>AMGSATISRRGILVIRHGERVDQVFGKSWLQQCTTADGKYYRPDLNFPRSLPRRSNGIKDFENDPPLSSCGIFQARLAGEALLDSGVRVTAVFASPALRCVQTAKHILEELKLEKKLKIRVEPGIFEWMKWEASKATLTFLTLEELKEANFNVDLDYRPALPRCSLMPAESYDQYVERCAVSMGQIINTCPQDMGITLIVSHSSALDSCTRPLLGLPPRECGDFAQLVRKIPSLGMCFCEENREDGKWDLVNPPVKTLTHGANSVFNWR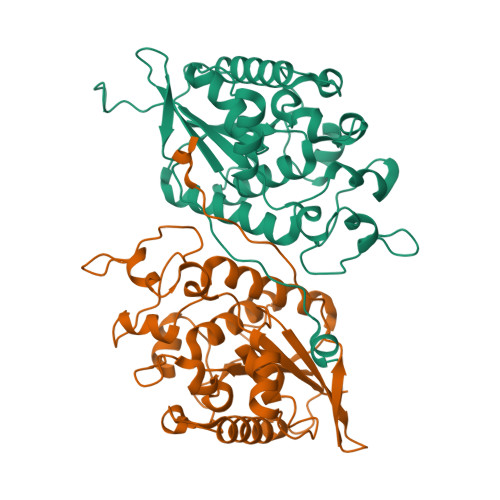NWIS[4x]>MTAHRSVLLVVHTGRDEATETARRVEKVLGDNKIALRVLSAEAVDRGSLHLAPDDMRAMGVEIEVVDADQHAADGCELVLVLGGDGTFLRAAELARNASIPVLGVNLGRIGFLAEAEAEAIDAVLEHVVAQDYRVEDRLTLDVVVRQGGRIVNRGWALNEVSLEKG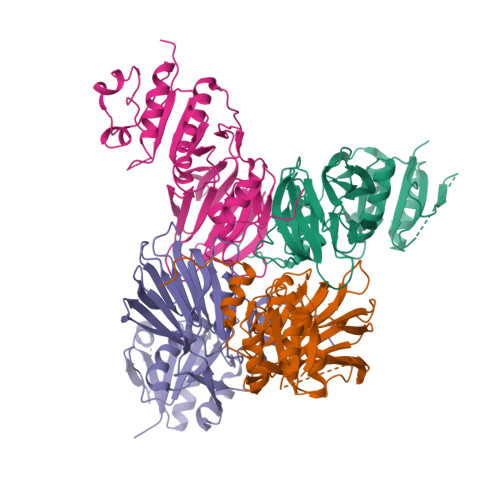PRLGVLGVVVEIDGRPVSAFGCDGVLVSTPTGSTAYAFSAGGPVLWPDLEAILVVPNNAHALFGRPMVTSPEATIAIEIEADGHDALVFCDGRREMLIPAGSRLEVTRCVTSVKWARLDSAPFTDRLVRKFRLPVTGWRGK[4x]>[6x]MGSSHHHHHHMKKARMTVDKDYKIAEIDKRIYGSFVEHLGRAVYDGLYQPGNSKSDEDGFRKDVIELVKELNVPIIRYPGGNFVSNYFWEDGVGPVEDRPRRLDLAWKSIEPNQVGINEFAKWCKKVNAEIMMAVNLGTRGISDACNLLEYCNHPGGSKYSDMRIKHGVKEPHNIKVWCLGNAMDGPWQVGHKTMDEYGRIAEETARAMKMIDPSIELVACGSSSKDMPTFPQWEATVLDYAYDYVDYISLHQYYGNKENDTADFLAKSDDLDDFIRSVIATCDYIKAKKRSKKDIYLSFDEWNVWYHSNNEDANIMQNEPWRIAPPLLEDIYTFEDALLVGLMLITLMKHADRIKIACLAQLINVIAPIVTERNGGAAWRQTIFYPFMHASKYGRGIVLQPVINSPLHDTSKHEDVTDIESVAIYNEEKEEVTIFAVN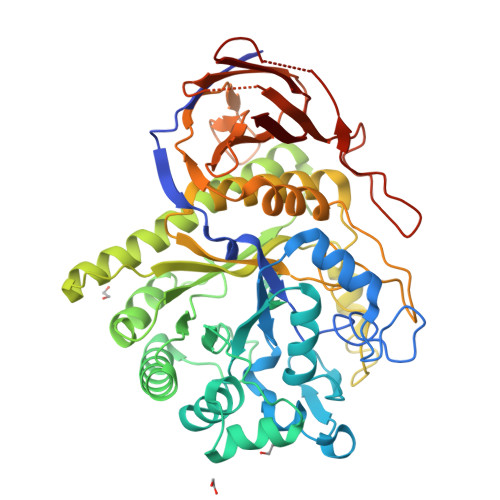RNIHEDIVLVSDVRGMKDYRLLEHIVLEHQDLKIRNSVNGEEVYPKNSDKSSFDDGILTSMLRRASWNVIRIGK> KKEDFVGHQVLRISVDDEAQVQKVKELEDLEHLQLDFWRGPARPGFPIDVRVPFPSIQAVKVFLEAHGIRYTIMIEDVQLLLDEEQEQMFASQGRARTTSTFNYATYHTLEEIYDFMDILVAEHPALVSKLQIGRSYEGRPIYVLKFSTGGSNRPAIWIDSGIHSREWITQASGVWFAKKITENYGQNSSFTAILDSMDIFLEIVTNPNGFAFTHSDNRLWRKTRSKASGSLCVGSDSNRNWDAGFG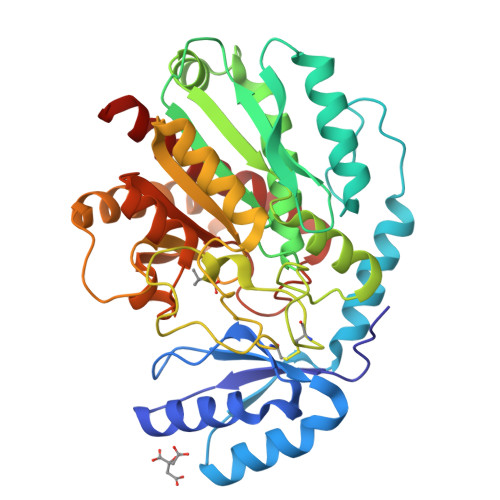GAGASSSPCAETYHGKYPNSEVEVKSITDFVKNNGNIKAFISIHSYSQLLLYPYGYKTQSPADKSELNQIAKSAVAALKSLYGTSYKYGSIITVIYQASGGVIDWTYNQGIKYSFSFELRDTGRRGFLLPASQIIPTAQETWLALLTIMEHTLNNS>[3x]XELKAIAQEFKAIAK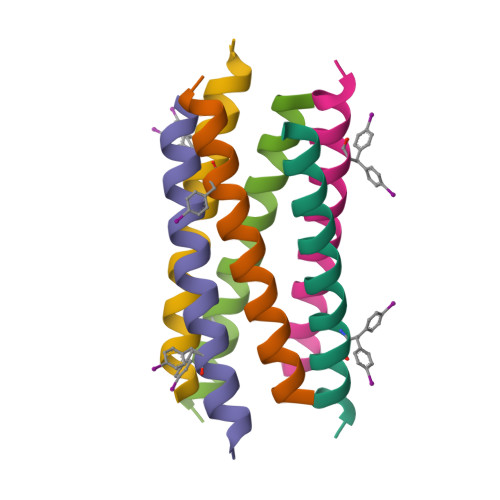EFKAIAFEFKAIAQKX JAK2, like other JAK family members, comprises a catalytically active C-terminal tyrosine kinase domain (JH1), a regulatory pseudokinase domain (JH2), and a Src homology-2 (SH2)-like domain that, together with the N-terminal FERM (N-terminal 4.1, ezrin, radixin, moesin) domain, forms the major receptor interaction moiety. The JH2 domain has a key role in mediating both negative and positive regulation of JAK kinase activity and numerous disease mutations locate in JH2, including the prevalent hyperactivating JAK2 V617F in MPN. Previous studies have demonstrated that JAK2 JH2 binds ATP and possesses regulatory autophosphorylation activity on Ser523 and Tyr570. To gain insights on the compound binding modes to JAK2 JH2 and to analyze whether any differences could be observed between binding to WT and V617F, we determined the crystal structures of selected small molecules with JAK2 JH2 WT and V617F.

Phenylpyrazolo-pyrimidone compounds 34, 35, and 36, analogs of hit 13, engaged JAK2 JH2 domain with selectivity over JH1. The compounds that targeted JH2 domain shared a trifluoro-group as R1. Diaminotriazole analog 18, diaminotriazine compounds 4 and 24, and phenylpyrazolo-pyrimidone analogs 34 and 36 targeted JAK2 JH2 with selectivity over JH1, although the affinity of these compounds to JH2 domain was micromolar and thus lower compared to the JH1-targeting compounds 1 and 2. All compounds bind to the hinge via three hydrogen bonds (H-bonds) with the exception of 36, which makes only one hydrogen bond to the backbone amide nitrogen of Val629. Since the compound binding does not induce significant changes in the ATP pocket, we compared the regions around residue 617 and the helix Cα between WT and V617F structures. It has been noted before that compound binding to JAK2 JH2 V617F can disrupt the aromatic packing of F617-F595-F594 and the conformation of F595 and F594 can be reverted back to the JAK2 JH2 WT conformation. In structures complexed with 6, 36, and 16, a WT-like conformation for the phenylalanines was observed. In the complexes with 36 and 16, the switch towards the WT-like conformation seems to start from the shifting of Gln626 gatekeeper position, which in turn affects the conformation of Leu624. This leucine forces both Phe594 and Phe595 to a new conformation. It appears to be possible to affect the conformation of the V617F region with small molecules, especially ones disturbing the position of the gatekeeper.

>[2x]VFHKIRNEDLIFNESLGQGTFTKIFKGVRREVGDYGQLHETEVLLKVLDKAHRNYSESFFEAASMMSKLSHKHLVLNYGVCFCGDENILVQEFVKFGSLDTYLKKNKNCINILWKLEVAKQLAAAMHFLEENTLIHGNVCAKNILLIREEDRKTGNPPFIKLSDPGISITVLPKDILQERIPWVPPECIENPKNLNLATDKWSFGTTLWEICSGGDKPLSALDSQRKLQFYEDRHQLPAPKAAELANLINNCMDYEPDHRPSFRAIIRDLNSLFTPDLVPRGSHHHHHH> MKIAGIDEAGRGPVIGPMVIAAVVVDENSLPKLEELKVRDSKKLTPKRREKLFNEILGVLDDYVILELPPDVIGSREGTLNEFEVENFAKALNSLKVKPDVIYADAADVDEERFARELGERLNFEAEVVAKHKADDIFPVVSAASILAKVTRDRAVEKL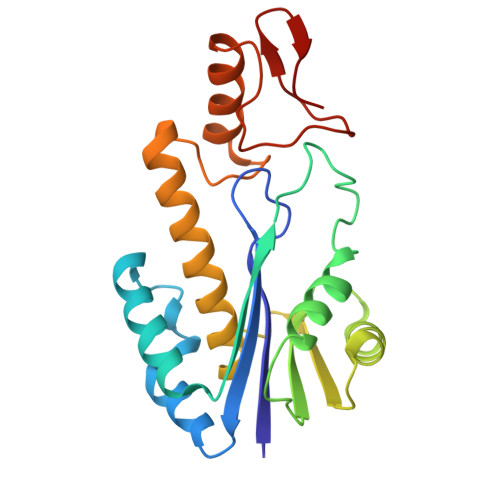KEEYGEIGSGYPSDPRTRAFLENYYREHGEFPPIVRKGAGAIIGLAVGGVVIA> KRAALIQNLRDSYTETSSFAVIEEWAAGTLQEIEGIAKAAAEAHGVIRNSTYGRAQAEKSPEQLLGVLQRYQDLCHNVYCQAETIRTVIAIRIPEHKEEDNLGVAVQHAVLKIIDELEIKTLGSGEKSGSG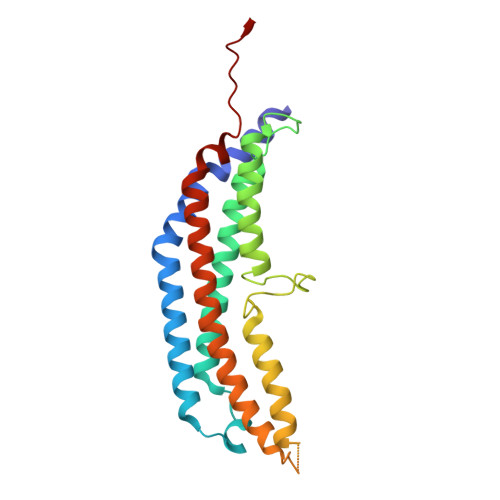GAPTPIGMYALREYLSARSTVEDKLLGSVDAESGKTKGGSQSPSLLLELRQIDADFMLKVELATTHLSTMVRAVINAYLLNWKKLIQPRTHLDVLYR>MGSSHHHHHHSQDPNSISTTMSSYSIQQSQKMLTQLQIDYATNTSSNTVVAYLHNVGETTISYLQNSVVYFGPNGQLQPVGYNSGSSPYWTVTSNSLQPGSKVKIIIYLSSPLSSNQYYTIQIVTPNGYTVSYMF[2x];>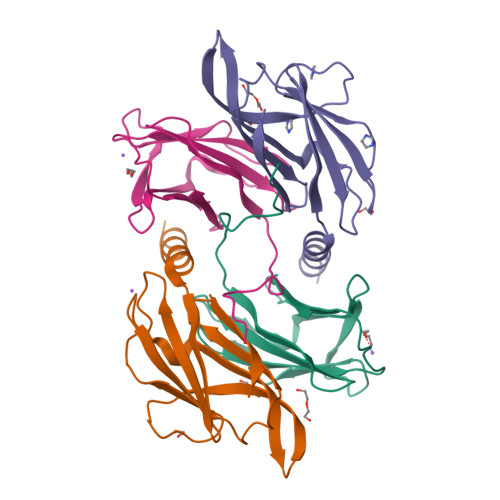MGSSHHHHHHSQDPNSNQAQELNHELELEQLETKITVSSVSLTGSTLNVVLENNGSTNLYDFQGFSVIVQYYANISNISTFNLSLYNYTKNSNPSPYYWTINTPLLAPGSQATLTIILPYPPYPNTQATVVIVTNYGPSVIWRGSL[2x]> PISPIETVPVKLKPGMDGPKVKQWPLTEEKIKALVEICTEMEKEGKISKIGPENPYNTPVFAIKKKDGTKWRKLVDFRELNKKTQDFWEVQLGIPHPAGLKKKKSVTVLDVGDAYFSVPLDEDFRKYTAFTIPSINNETPGIRYQYNVLPQGWKGSPAIFQSSMTKILEPFRKQNPDIVIYQYMDDLYVGSDLEIGQHRTKIEELRQHLLRWGLTTPDKKHQKEPPFLWMGYELHPDKWTVQPIVLPEKDSWTVNDIQKLVGKLNWASQIYPGIKVRQLCKLLRGTKALTEVIPLTEEAELELAENREILKEPVHGVYYDPSKDLIAEIQKQGQGQWTYQIYQEPFKNLKTGKYARMRGAHTNDVKQLTEAVQKITTESIVIWGKTPKFKLPIQKETWETWWTEYWQATWVPEWEFVNTPPLVKLWYQLEKEPIVGAETFYVDGAASRETKLGKAGYVTNKGRQKVVTLTDTTNQKTELQAIHLALQDSGLEVNIVTASQYALGIIQAQPDQSESELVNQIIEQLIKKEKVYLAWVPAHKGIGGNEQVDKLVSAGIRKIL;> MRGSHHHHHHGSQLPISPIETVPVKLKPGMDGPKVKQWPLTEEKIKALVEICTEMEKEGKISKIGPENPYNTPVFAIKKKDGTKWRKLVDFRELNKKTQDFWEVQLGIPHPAGLKKKKSVTVLDVGDAYFSVPLDEDFRKYTAFTIPSINNETPGIRYQYNVLPQGWKGSPAIFQSSMTKILEPFRKQNPDIVIYQYMDDLYVGSDLEIGQHRTKIEELRQHLLRWGLTTPDKKHQKEPPFLWMGYELHPDKWTVQPIVLPEKDSWTVNDIQKLVGKLNWASQIYPGIKVRQLCKLLRGTKALTEVIPLTEEAELELAENREILKEPVHGVYYDPSKDLIA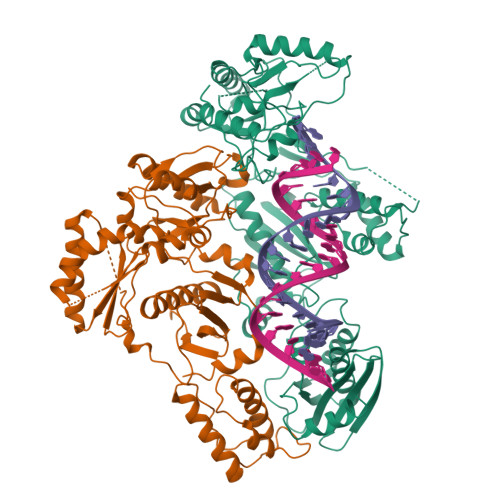EIQKQGQGQWTYQIYQEPFKNLKTGKYARMRGAHTNDVKQLTEAVQKITTESIVIWGKTPKFKLPIQKETWETWWTEYWQATWVPEWEFVNTPPLVKLWYQLEKEPIVGAETF To gain more information regarding the dynamics of the OMF tunnelling mechanism, we focused our interest on OprN, the OMF protein associated with the MexEF complex within P. aeruginosa. This efflux pump is implicated in the resistance to fluoroquinolones, the most used antibiotic class. As a representative member of the OMF family, OprN structure shows two main domains: a channel of 100 Å long located in the periplasm, also known as the α-domain, and a β-barrel of 30 Å long inserted in the outer membrane. The protein channel is closed by a lid of three β-turns at the extracellular side and occluded by a constriction of three a-coiled-coils at the periplasmic side, which gating mechanism is probably ruled by an iris-like movement.

Although OprN has only a moderate degree of homology with OprM (31.4%), its structure was solved by Molecular Replacement with OprM X-ray structure. The assembly of three monomers results in a long and wide tunnel responsible for the transport of drug out of the bacteria. In addition, an equatorial domain called the buoy domain, mainly composed of α-helices and flexible loops is located in the middle of the α-domain. Surprisingly, this buoy domain is the main structural feature that differs among the OMFs proteins, both in structure and sequence. At the N-terminus Cys residue, it was possible to construct at each monomer the acyl group of the post-translational palmitoylation. Although difficult to observe due to some disorder, 4 to 10 carbons of the aliphatic chains of the different palmitoyl were built. We also observed a dual acylation at the same modified cysteine, an unusual post-translational lipidation in the OMF family. OprN-wt and OprN-Xe structures perfectly match each other with a Cα rms deviation of 0.21 Å over 1352 atoms of the trimer, suggesting an overall protein fold unaffected by the xenon interaction. The main differences are limited to the C-terminus orientation as well as the distribution of the detergent and additive molecules around the trimer.

>CTVGPDYRTPDTAAAKIDATASKPYDRSRFESLWWKQFDDPTLNQLVEQSLSGNRDLRVAFARLRAARALRDDVANDRFPVVTSRASADIGKGQQPGVTEDRVNSERYDLGLDSAWELDLFGRIRRQLESSDALSEAAEADLQQLQVSLIAELVDAYGQLRGAQLREKIALSNLENQKESRQLTEQLRDAGVGAELDVLRADARLAATAASVPQLQAEAERARHRIATLLGQRPEELTVDLSPRDLPAITKALPIGDPGELLRRRPDIRAAERRLAASTADVGVATADLFPRVSLSGFLGFTAGRGSQIGSSAARAWSVGPSISWAAFDLGSVRARLRGAKADADAALASYEQQVLLALEESANAFSDYGKRQERLVSLVRQSEASRAAAQQAAIRYREGTTDFLVLLDAEREQLSAEDAQAQAEVELYRGIVAIYRSLGGGWQPSAHHHHHH[3x]> SNAMIPFNAPPVVGTELDYMQSAMNSGKLC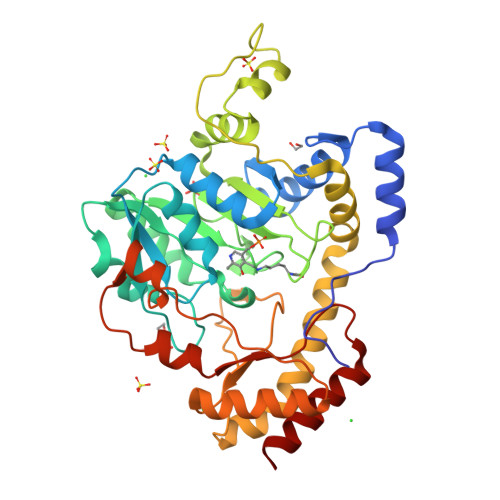GDGGFTRRCQQWMEQRFGTAKALLTPSCTASLEMAALLLDIQPGDEVIMPSYTFVSTANAFVLRGAKIVFVDIRRDTMNIDETLIEAAITDKTRAIVPVHYAGVACEMDTIMAIADKYNLFVVEDAAQGVMSTYKGRALGTIGHIGCFSFHETKNYTAGGEGGATLINDRTLVERAEIIREKGTNRSQFFRGLVDKYTWRDIGSSYLMSDLQAAYLWAQLEAAERINQQRLALWQNYYDALLPLARAGRIELPTVPADCGQNAHMFYIKLRDIEDRSRLIAWLKEAEILAVFHYIPLHSCPAGEQFGEFRGEDRYTTQESERLVRLPLFYNLSVVNQRTVINSLLSYFS>MVAVEQSEASRLGPVFDSCRANNRAALIGYLPTGYPDVPASVAAMTALVESGCDIIEVGVPYSDPVMDGPTIARATEAALRGGVRVRDTLAAVEAISIAGGRAVVMTYWNPVLRYGVDAFARDLAAAGGLGLITPDLIPDEAQQWLAASEEHRLDRIFLVAPSSTPERLAATVEASRGFVYAASTMGVTGARDAVSQAAPELVGRVKAVSDIPVGVGLGVRSRAQAAQIAQYADGVIVGSALVTALTEGLPRLRALTGELAAGVRLGMSAHHHHHH[4x];>MSAAIAEPTSHDPDSGGHFGGPSGWGGRYVPEALMAVIEEVTAAYQKERVSQDFLDDLDRLQANYAGRPSPLYEATRLSQHAGSARIFLKREDLNHTGSHKIN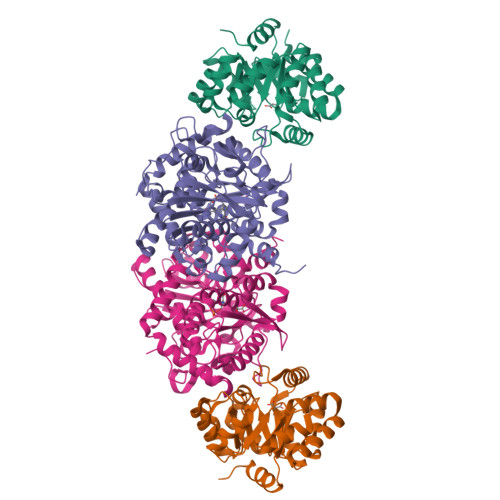NVLGQALLARRMGKTRVIAETGAGQHGVATATACALLGLDCVIYMGGIDTARQALNVARMRLLGAEVVAVQTGSKTLKDAINEAFRDWVANADNTYYCFGTAAGPHPFPTMVRDFQRIIGMEARVQIQGQAGRLPDAVVACVGGGSNAIGIFHAFLDDPGVRLVGFEAAGDGVETGRHAATFTAGSPGAFHGSFSYLLQDEDGQTIESHSISAGLDYPGVGPEHAWLKEAGRVDYRPITDSEAMDAFGLLCRMEGIIPAIESAHAVAGALKLGVELGRGAVIVVNLSGRGDKDVETAAKWFGLLGND[4x]>[8x]MGSSHHHHHHSSGEQKLISEEDLSSGENLYFQGHMASSTSLPAPGSRPKKPLGKMADWFRQTLLKKPKKRPNSPESTSSDASQPTSQDSPLPPSLSSVT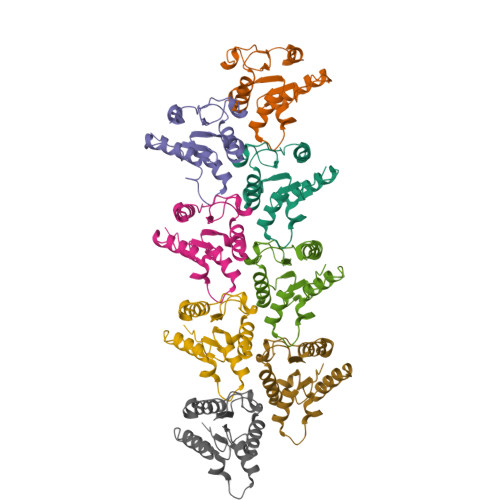SPSLPPTHASDSGSSRWSKDYDVCVCHSEEDLVAAQDLVSYLEGSTASLRCFLQLRDATPGGAIVSELCQALSSSHCRVLLITPGFLQDPWCKYQMLQALTEAPGAEGCTIPLLSGLSRAAYPPELRFMYYVDGRGPDGGFRQVKEAVMRYLQTLS> MASSHNVLMRLVASAYSIAQKAGTIVRCVIAEGDLGIVQKTSATDLQTKADRMVQMSICSSLSRKFPKLTIIGEEDLPPGEVDQELIEDGQSEEILKQPCPSQYSAIKEEDLVVWVDPVDGTKEYTEGLLDNV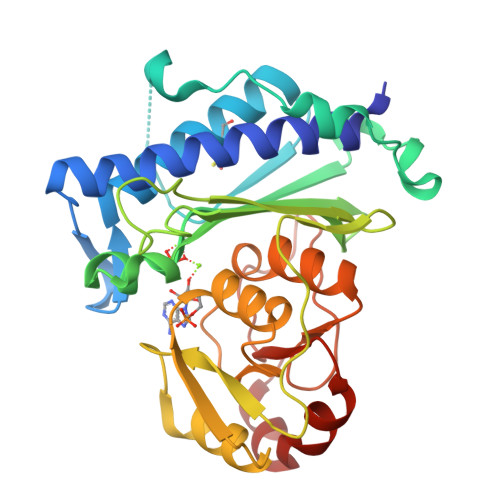TVLIGIAYEGKAIAGIINQPYYNYQAGPDAVLGRTIWGVLGLGAFGFQLKEAPAGKHIITTTRSHSNKLVTDCIAAMNPDNVLRVGGAGNKIIQLIEGKASAYVFASPGCKKWDTCAPEVILHAVGGKLTDIHGNPLQYDKEVKHMNSAGVLAALRNYEYYASRVPESVKSALIP>[2x]AMADITSLYKKAGSAAAPFAYNSAGEPPVSRRSFPKGFIFGTASSSYQYEGGAAEGGRGPSIWDTFTHQHPEKIADRSNGDVASDSYHLYKEDVRLMKDMGMDAYRFSISWTRILPNGSLRGGVNKEGIKYYNNL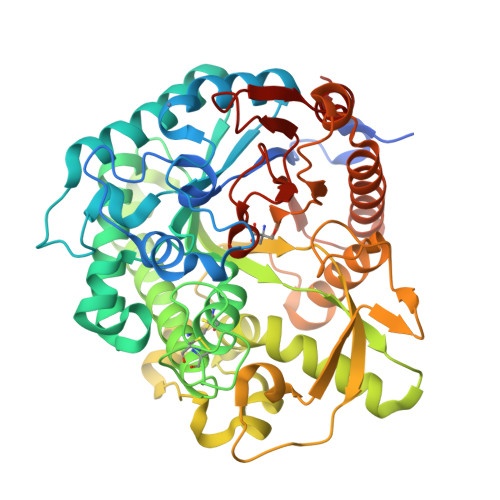INELLSKGVQPFITLFHWDSPQALEDKYNGFLSPNIINDFKDYAEICFKEFGDRVKNWITFNEPWTFCSNGYATGLFAPGRCSPWEKGNCSVGDSGREPYTACHHQLLAHAETVRLYKAKYQALQKGKIGITLVSHWFVPFSRSKSNNDAAKRAIDFMFGWFMDPLIRGDYPLSMRGLVGNRLPQFTKEQSKLVKGAFDFIGLNYYTANYADNLPPSNGLNNSYTTDSRANLTGVRNGIPIGPQAASPWLYVYPQGFRDLLLYVKENYGNPTVYITENGVDEFNNKTLPLQEALKDDARIEYYHKHLLSLLSAIRDGANVKGYFAWSLLDNFEWSNGYTVRFGINFVDYNDGRKRYPKNSAHWFKKFLLK> MRKIQVGVTGMTCAACSNSVEAALMNVNGVFKASVALLQNRADVVFDPNLVKEEDIKE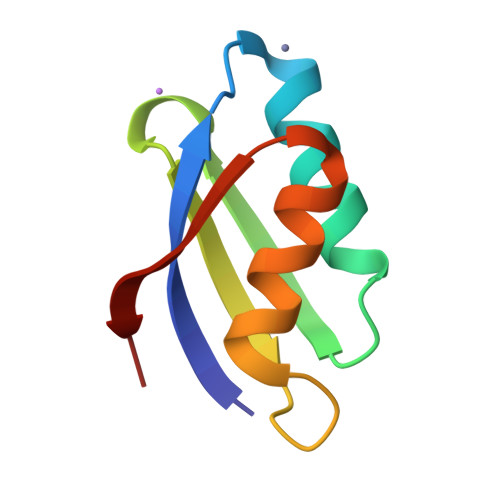EIEDAGFEAEILAEEW> SMKDVPDSQQHPAPEKSSKVSEQLKCCSGILKEMFAKKHAAYAWPFYKPVDVEALGLHDYCDIIKHPMDMSTIKSKLEAREYRDAQEFGADVRLMFSNCYKYNPPDHEVVAMARKLQDVFEMRFAKMPDE

Bromodomains (BRDs) are protein interaction modules that specifically recognize ε-N-lysine acetylation motifs, a key event in the reading process of epigenetic marks. The 61 BRDs in the human genome cluster into eight families based on structure/sequence similarity. Despite large sequence variations, all BRD modules share a conserved fold that comprises a left-handed bundle of four α helices (αZ, αA, αB, αC), linked by loop regions of variable length (ZA and BC loops), which line the Kac binding site and determine binding specificity. The four helices form a deep cavity that is extended by the two loop regions (ZA and BC loops), creating a largely hydrophobic Kac binding pocket.

For instance, BRD4(2) did not interact with H3 peptides singly acetylated on K4. In contrast, this domain showed strong interaction with diacetylated H3 (H3K4acK9ac) but not with the same peptide acetylated at K4 but trimethylated at K9 (H3K4acK9me3). The strongest interaction was observed using diacetylated H3K4acK9ac in combination with phosphorylation at T3. Screening against BRDs of the BET family showed that BRD4(2) interacted with most combinations of two and three acetylated lysines, whereas BRD4(1) seemed to specifically recognize multiple marks found on the H4 tail. The second BET BRDs bound to tetra-acetyl H4 peptides with about 10-fold weaker affinities, suggesting that the first BRD in BET proteins recognizes the H4 tail. In contrast, the second BRDs of BET BRDs bound either weakly (BRD2), not at all (BRD3), or promiscuously (BRD4) to histone sequences and their variants present in this array. In contrast, diacetylation had only a modest effect on binding affinities of the second BRD of BRD4. As reported for interactions with single acetylation sites in the case of the BRDs of BRD2 (Umehara et al., 2010), alanine mutants of the conserved asparagine (N140 and N443 in the first and second BRDs in BRD4) did also abolish binding of diacetylated peptides in both SPOT assays as well as in ITC. Similarly, our array and ITC studies on BRD4 showed that the first BRD of this protein has high affinity for the histone H4 tail, whereas the second BRD most likely recognizes multiply acetylated marks in histone H3.>MKPYQRQFIEFALNKQVLKFGEFTLKSGRKSPYFFNAGLFNTGRDLALLGRFYAEALVDSGIEFDLLFGPAYKGIPIATTTAVALAEHHDKDLPYCFNRKEAKDHGEGGSLVGSALQGRVMLVDDVITAGTAIRESMEIIQAHGATLAGVLISLDRQERGRGEISAIQEVERDYGCK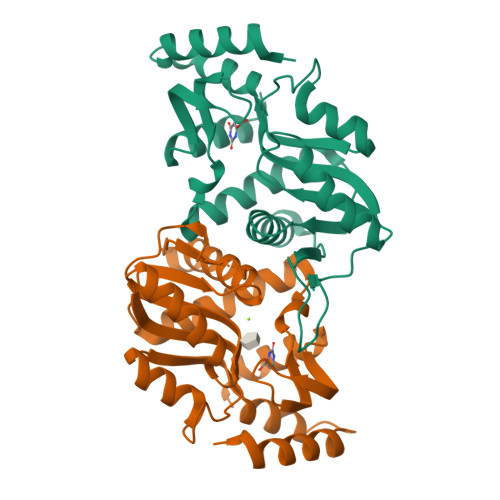VISIITLKDLIAYLEEKPDMAEHLAAVRAYREEFGV[2x]2-[4-(4-methoxyphenyl)piperazine-1-carbonyl]-5lambda~6~-thieno[3,2-c][1]benzothiopyran-5,5(4H)-dione 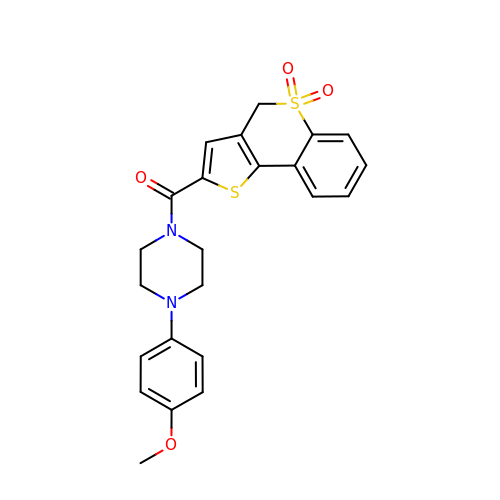| C23 H22 N2 O4 S2 | YVIJPELUPZUEJX-UHFFFAOYSA-N> MSNGDWGQSQRTRGTGPVRGIRTMDVNAPGGGSGGSALRILGTASCNQAHCKFGRFAGIQCVSNCVLYLVKSFLAGRPLTSRPELDEVLDEGARLDALMRQSGILKGHEMAQLTDVPSSVVLRGGGRVHIYRSAEIFGLVLFPAQIANSAVVQSLAEVLHGSYNGVAQFILYICDIYAGAIIIETDGSFYLFDPHCQKDAAPGTPAHVRVSTYAHDILQYVGAPGAQYTCVHLYFLPEAFETEDPRIFMLEHYGVYDFYEANGSGFDLVGPELVSSDGEAAGTPGADSSPPVMLPFERRIIPYNLRPLPSRSFTSDSFPAARYSPAKTNSPPSSPASAAPASAAPASAAPASAAPASAAPASAAPASAAPASAAPASSPPLFIPIPGLGHTPGVPAPSTPPRASSGAAPQTPKRKKGLGKDSPHKKPTSGRRLPLSSTTDTEDDQLPRTHVPPHRPPSAARLPPPVIPIPHQSPPASPTPHPAPVSTIAPSVTPSPRLPLQIPIPLPQAAPSNPKIPLTTPSPSPTAAAAPTTTTLSPPPTQQQPPQSAAPAPSPLLPQQQPTPSAAPAPSPLLPQQQPPPSAARAPSPLPPQQQPLPSATPAPPPAQQLPPSATTLEPEKNHPPAADRAGTEISPSPPFGQQPSFGDDASGGSGLVRYLSDLEEPFLSMSDSEEAESDLASDIPTTEDEDMFEDEVFSNSLESGSSAPTSPITLDTARSQYYQTTFDIETPEMDFVPLESNIARIAGHTYQEQAIVYDPASNREVPEADALSMIDYLLVTVVLEQGLIRSRDRSSVLNLLEFLKDWSGHLQVPTLDLEQLLTSELNIQNLANMLSENKGRAGEFHKHLAAKLEACLPSLATKDAVRVDAGAKMLAEIPQLAESDDGKFDLEAARRRLTDLLSGGDQEAGEGGGEPEDNSIYRGPHVDVPLVLDDESWKRLLSLAEAARTAVARQQAGVDEEDVRFLALLTAIEYGAPPAASVPPFVHNVAVRSKNAALHVRRCTADIRDKVASAASDYLSYLEDPSLPTVMDFDDLLTHLRHTCQIIASLPLLNIRYTSIEWDYRELLYLGTALSDMSGIPWPLERVEEDDPSIAPLPEFETVAKKQKELETTRENEKRLRTILDDIEAMLGLAGVASAPGAPISPASPSATPANHDNPEATPPLADTAALTIPVIEKYIANAGSIVGAAKNPTYIRLRDTIQQIVRSKKYLMNILKSITFYTIDNYIASFEESIDHLYRDLPVLDPEVQDGIDRILDPMVSEALHTFEMGNRLTLEPARLVALQNFATHSTLKETAAAVNLLPGLLAVYDATITGQAPEDALRLLSGLQNQLSQTLIPGKLKKRFLSYLQKLKNNNNDQLRQKEVQAWRLEAEGFKPATEEQLEAFLDTAPNKELKRQYEKKLRQLMETGRKEKEKLREQEDKERQERRAREANEAWARIRKALGARPEPAPTSPDDWNTLLASLLPDNTDSAAAAAAAVARNTDILDSLTQILAAMLLGITRVRRERLRSLLVDDGGAAERMEAAEPGWFTDIETGPLARLDAWPATPAATAKEGGGGRGAEEAAGALFRARTAADAIRSALAQTRQALQSPDMKSAVVNTDLEAPYAEYERGLAGLLEKRRAAEAALTAIVSEYVDRTLPEATNDPGQANLPPPPTIPQATAPPRLASDSALWPKKPQLLTRRERDDLLQATGDFFSELLTEAEAAEVRALEEQVRESQTLMAKAHEMAASTRRGFHTALEAVLSRSRDEAPDDELRSLLPSPPKAPVQAPLEAALARAAAGNGSWPYRKSLAAAKWIRGICEAVRGLSEGALALAGGAGAWLNLAAAADGEIHELTRLLEVEGMAQNSMDGMEELRLALATLDPKRVAGGKETVADWKRRLSRLEAIIQEAQEESQLQGTLQDLVTQARGHTDPRQLKIVVEAARGLALGASAGSQYALLKDKLLRYASAKQSFLAFYETAQPTVFVKHPLTNNLPLLITISAPPTGWGNGAPTRRAQFLAAAGPAKYAGTLWLETESPCDPLNPAYVSADTQEPLNYIPVYHNFLEYVMPTVLENPEAFSLTPAGRPQAIGPPQDDQERRRRTLASVASARLSAAAADSYWDTWPDVESNAGELLREYVSAPKALMEDLADNPIVAMTLLAHASLIASRNHPPYPAPATDREVILLEQREMMALLVGTHPAYAAAFLGAPSFYAGLGLVSALARDGGLGDLLSDSVLTYRLVRSPASGRGGMPSTTRGSNDGEDARRLTRHRIAGPPTGFIFFQDAWEEMDTRAALWPHPEFLGLVHNQSTARARACMLLLARRCFAPEALQQLWHSLRPLEGPVAFQDYLRDFVKQAYTRGEELPRAEGLEVPRETPSSYGTVTGRALRNLMPYGTPITGPKRGSGDTIPVSVFEAAVAAAFLGRPLTLFVSSQYLFNLKTLGQVRVVAPLLYCDGHSEPFRSLVETISLNFLQDLDGYSESFEPEMSIFARQAVWLRELLTEARAAKPKE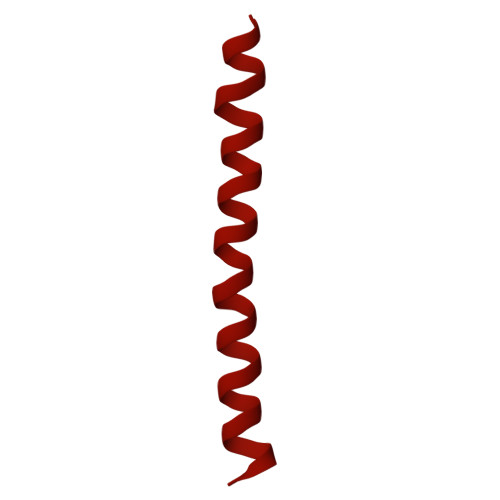ARPPTVAILANRKNIIWKCFTYRHNLPDVQFYFNAAGASRWPTDVLNPSFYEHEDPPLPVGYQLPPNPRNVQELFSGFPPRVGHGLVSGDGFQSADNTPASSDRLQQLGGGETDQGEKGSTTAESEASGPPSPQSPLLEKVAPGRPRDWLSPTSSPRDVTVTPGLAAPITLPGPRLMARPYFGAETRASESPDRSPGSSPRPWPKDSLELLPQPAPQQPPSSPWASEQGPIVYTLSPHSTPSTASGSQKKHTIQIPGLVPSQKPSYPPSAPYKPGQSTGGIAPTPSAASLTTFGLQPQDTQASSQDPPYGHSIMQREKKQQGGREEAAEIRPSATRLPTAVGLRPRAPVVAAGAAASATPAFDPGEAPSGFPIPQAPALGSGLAAPAHTPVGALAPRPQKTQAQRPQDAAALPTPTIKAVGARPVPKATGALAAGARPRGQPTAAPPSAASPPRVSLPVRSRQQQSPAIPLPPMHSGSEPGARPEVRLSQYRHAGPQTYTVRKEAPPSAASQLPKMPKCKDSMYYPPSGSARYPAPFQALSFSQSVASPAPSSDQTTLLWNTPSVVTQFLSIEDIIREVVTGGSTSGDLVVPSGSPSSLSTAAPEQDLRYSLTLSQASRVLSRFVSQLRRKLERSTHRLIADLERLKFLYL MICAL1, identified as a Molecule Interacting with CasL, belongs to the family of MICAL proteins, conserved from insects to humans. MICALs are intracellular proteins that catalyse oxidation–reduction (redox) reactions through their flavoprotein monooxygenase (MO) domain and use F-actin as a substrate. These enzymes bind flavin adenine dinucleotide (FAD)2627 and use the coenzyme nicotinamide adenine dinucleotide phosphate (NADPH) and O2 in redox reactions, causing disassembly of F-actin likely by directly oxidizing specific actin methionines. Active, GTP-bound Rab35 directly interacts with the tail of MICAL1 through a flat three-helix domain revealed by X-ray crystallography.

The interaction with Rab35 required the last 150 residues of MICAL1 (aa 918–1067), in which the last 41 residues are essential. The C-terminal region of MICAL1 has been described as comprising segments of coiled-coils2137, potentially implying oligomerization of this enzyme2137. We determined a structure of this domain by X-ray crystallography at 3.3 Å resolution. Surprisingly, the structure consists of a curved sheet of three helices, exposing two opposite flat surfaces, which differs from most three helices folds that usually form compact bundles. This structure is formed by anti-parallel intramolecular coiled-coils interactions: while the first part of helix H2 makes coiled-coil interactions with helix H1, the second part of helix H2 interacts with helix H3 also with coiled-coil interactions, and no interactions are formed between the H1 and H3 helices. Biophysical measurements by MALS and SAXS indicated that this domain is a monomer, and thus does not form an elongated dimeric coiled-coil, as previously found for other Rab-effectors4647. Overall, the domain of ∼80 × 30 Å in dimension exposes two large curved surfaces on either side of the helices. The mutant S2 (R1012E, M1015R, L1034K and V1038E) and the single mutant M1015R had very low binding affinity to Rab35 indicating that both H2 and H3 helices participate in Rab35 binding, while the opposite face of the three helical domain defined by the S1 mutations do not participate in Rab35 binding. Most of these residues are conserved among MICAL proteins, consistent with Rab-binding properties of several MICAL family members and with the crystal structure of Rab1 bound to MICAL-cL48. This Rab35-binding surface (oval in Fig. 5c) explains why the Δ41 fragment (aa 918–1026), which lacks the whole H3 helix, is unable to bind Rab35 (see above). Importantly, we reveal that Rab35 activates the enzymatic activity of MICAL1 by displacing the inhibitory intramolecular interaction between the C-terminus of MICAL and its catalytic monooxygenase domain.

> KEEEMKRFCKAQTIQRRLNEIEAALRELEAEGVKLELALRRQSSSPEQQKKLWVGQLLQLVDKKNSLVAEEAELMITVQELNLEEKQWQLDQELRGYMNREENLKTAADRQAEDQVLRKLVDLVNQRDALIRFQEERRLSELALGTGAQG>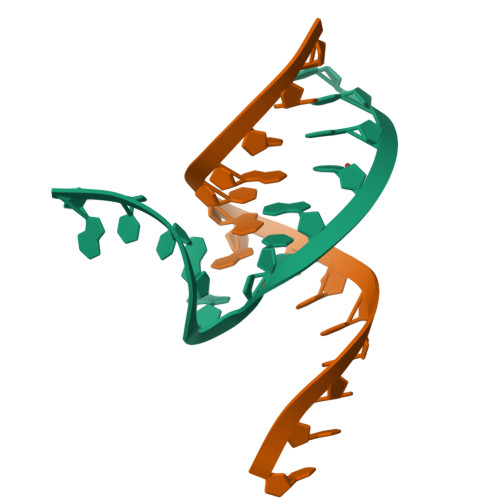 CGAUCCUAGUGUGG;> CCAUGCGAACCG(1R,3R,7E,17beta)-17-{(1S,2E,5R)-5-hydroxy-1-methyl-5-[(3S,5S,7S)-tricyclo[3.3.1.1~3,7~]dec-1-yl]pent-2-en-1-yl}-2-methylidene-9,10-secoestra-5,7-diene-1,3-diol 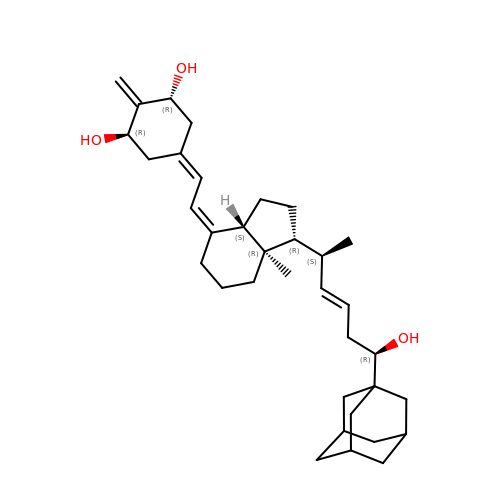| C35 H52 O3 | MOSWJCBKXGNCIG-HBOJQGNGSA-N Mutations in the mitochondrial aminoacyl‐tRNA synthetases (mtaaRSs) can cause profound clinical presentations, and have manifested as diseases with very selective tissue specificity. Among the recently reported pathogenic variants are point mutations in FARS2 gene, encoding the human mitochondrial PheRS. Patient symptoms range from spastic paraplegia to fatal infantile Alpers encephalopathy. How clinical manifestations of these mutations relate to the changes in three‐dimensional structures and kinetic characteristics remains unclear, although impaired aminoacylation has been proposed as possible etiology of diseases.

Here, we report four crystal structures of HsmtPheRS mutants, and extensive MD simulations for wild‐type and nine mutants to reveal the structural changes on dynamic trajectories of HsmtPheRS. Using steady‐state kinetic measurements of phenylalanine activation and tRNAPhe aminoacylation, we gained insight into the structural and kinetic effects of mitochondrial disease‐related mutations in FARS2 gene.

> PGSVVELLGKSYPQDDHSNLTRKVLTRVGRNLHNQQHHALWLIKERVKEHFYKQYVGRFGTPLFSVYDNLSPVVTTWQNFDSLLIPADHPSRKKGDNYYLNRTHMLRAHTSAHQWDLLHAGLDAFLVVGDVYRRDQIDSQHYPIFHQLEAVRLFSKHELFAGIKDGESLQLFEQSSRSAHKQETHTMEAVKLVEFDLKQTLTRLMAHLFGDELEIRWVDCYFPFTHPSFEMEINFHGEWLEVLGCGVMEQQLVNSAGAQDRIGWAFGLGLERLAMILYDIPDIRLFWCEDERFLKQFCVSNINQKVKFQPLSKYPAVINDISFWLPSENYAENDFYDLVRTIGGDLVEKVDLIDKFVHPKTHKTSHCYRITYRHMERTLSQREVRHIHQALQEAAVQLLGVEGRF>GEVSYAKERVRLITASGRTHDLTVELAVD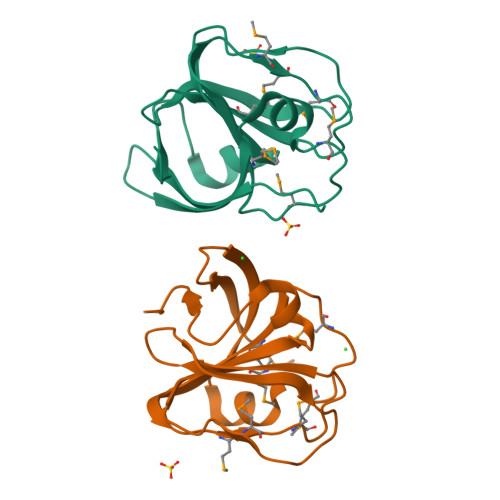PSQREQGLMYRRQMAPDHGMLFDFGETRPVMMWMKNTYLPLDMLFIASDGTIRTIHENAVPHSEAIIDSREPVAYVLELNAGTVKRLGVSPGDRLEGAGLPATKRAN[2x]>[4x]MKVEEILEKALELVIPDEEEVRKGREAEEELRRRLDELGVEYVFVGSYARNTWLKGSLEIDVFLLFPEEFSKEELRERGLEIGKAVLDSYEIRYAEHPYVHGVVKGVEVDVVPCYKLKEPKNIKSAVDRTPFHHKWLEGRIKGKENEVRLLKGFLKANGIYGAEYKVRGFSGYLCELLIVFYGSFLETVKNARRWTRRTVIDVAKGEVRKGEEFFVVDPVDEKRNVAANLSLDNLARFVHLCREFM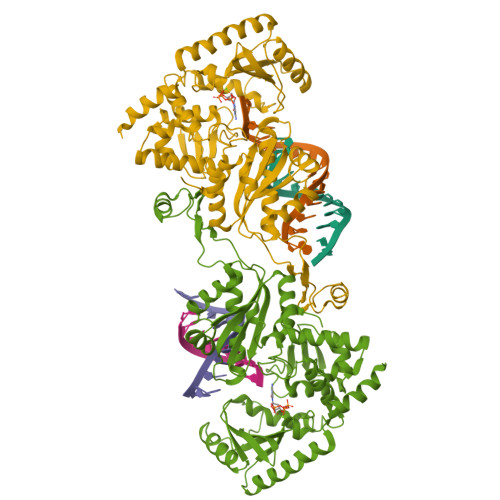EAPSLGFFKPKHPLEIEPERLRKIVEERGTAVFAVKFRKPDIVDDNLYPQLERASRKIFEFLERENFMPLRSAFKASEEFCYLLFECQIKEISRVFRRMGPQFEDERNVKKFLSRNRAFRPFIENGRWWAFEMRKFTTPEEGVRSYASTHWHTLGKNVGESIREYFEIISGEKLFKEPVTAELCEMMGVKD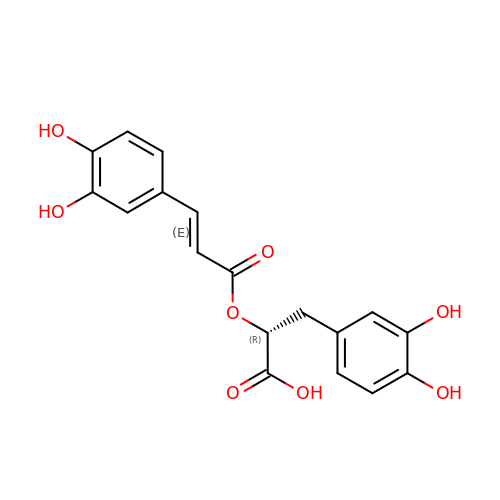(2R)-3-(3,4-dihydroxyphenyl)-2-{[(2E)-3-(3,4-dihydroxyphenyl)prop-2-enoyl]oxy}propanoic acid | C18 H16 O8 | DOUMFZQKYFQNTF-WUTVXBCWSA-N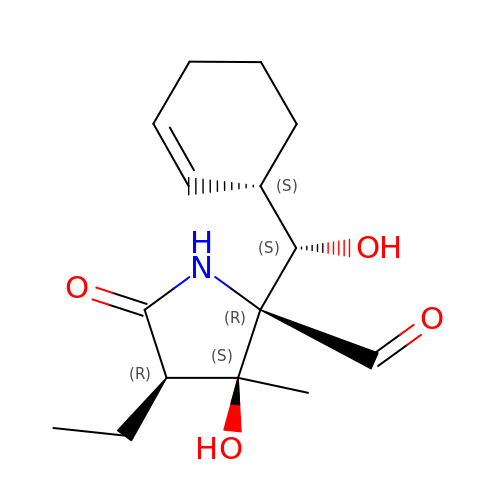(2R,3S,4R)-2-[(S)-(1S)-cyclohex-2-en-1-yl(hydroxy)methyl]-4-ethyl-3-hydroxy-3-methyl-5-oxopyrrolidine-2-carbaldehyde | C15 H23 N O4 | HSXZBJZQFUJQNN-FUQNVFFISA-N> MIIINKNNDKKSLFLLLVSLIFVLFVSNVIADTDYAISPVSLLLPYSTSKYRKPYKLEANKGCFEWINTNPDLVEITPLYESAASCSPSSNDKQQNIGAPDLSLWDNSLNQPNKKCSKAVLVSVRSGTVSERNSAFIYAEEQVTGKKLQCEVFVDRISSIVIETTTKTMYKDDLEELHVRAYDSVGNVFSSIIGLEFEWSITSGNIIQIVPFRGFPLDDVALKMEQESLQTSFVLVQGVDTGRTEINTKLTEPTYKDIQHSTTISILEPLQLNPSYLLYVIPGTQIQYQLLTKKRNILENIPLPNPNYIWSSSNSKVGKVDNSGNFMALDLGRTDLKVQHKNMSDNKVQAFVNVVHPSYLAIKIEPLKSGLGPVSNWNLIENRDYILVVELYDASGHKIHSSEITFDLNIPTEYFERLPSSQIPPNTPKRSDTFYLKAIKQGLVALKASLVKVYDLNLKKYTQLLNPISVEQEVTIHSQIQLSPPIVYLPYLPNHRQYSMIRPIGGSGEYNWYTNNSAIVTVDPTGAITSQTSSGQTEVIVVDKKNPHNRDKVLVIVLQPDEIIITPSQVEVQVGQTLKLSTQLLSKQLSKGVHFDSCNLDDLEWRVDDSNANNDNNGGGGSNQERSFSLLPLQKTNTPKKEQPDLCSTREFLAIKEGSNVISVSYMGMRAKILIFAYPPLKSDQSEILLTLGSTLNVFFSGGPEPWHLERKSHFQSIVSNLTNEQNVLSIVPGNGNSFRVTCLTHTNPSKPIGIELTIGNKVTTTNPYPASPSITIPYSCRPPASIQLQVANLPKDHQIQDSSHHQQIQQQEQQQQQQQQQSTCQDTIFSIKKQKQGEIGTYKIRNDRDIPFIAQVFDDNGKPFTNYSSLVFDWKSSDQTQAKWLRDYNQNDHLSTLSLSKEQGKVIITVSILGYDQELLRQNKIRSSDLDTSKLVSSLELHLLSSVVLFPDYYTMYLNDKNHLKIEAIGGSKNFAFTSNNSKIASLSYQPNSDFVTVIPNQQGYLKVEVRDICLGSDNNKDQQQQYQQKQQKHQQQQQSNTSPSIVQISEVHSIELDVQDMVQVGDSINLIVKGFSQNGQQFDSTQY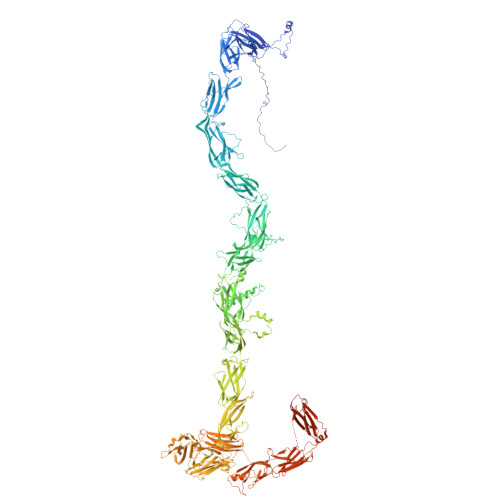QYMNIIPHIDNPNVLSMTQSSDSQVFTLKGLDQGLVTLSVTIQNPKTSFSATSKTIQIQVFPPFRVSPSVLHLVPGGHFQIHWTGGAPIRQDVSFVSSDPSIVNLSGREDLVGELVALKVGEATIKAIAQIVDPITGKKTIIGEDKLMVYVKNMTGIRIHSSINKILVGNEAKLRVVGANGETPFTYGTVDLFFKWECLDSNIATLLPIYERANTTVEAEGSFSVRVMGKNAGSTSITVWAYSGGDKTKHLFQAASLQINVIPDIPIQTTSLLLPLNTPSSFIVNNHLDKTGIEFYPLMDGHGSSSCKDVIDIGDNKIVSLDKIGTCYVSAVRDGRMDTSKLFKINSKPFSHLELLPINPTSTVIPIGGSMSFAIYLRDDIGEVFTEYGSSAIFSSEVSNTGIISSSIDANVVTIKGIRAGLVTLHVYLKDMPHLDDYIKIFVGRLVEPHQPILHVGSMITFSIAKDQLEQRGFSLPSSDEKVWSSGDPSILQVDPITGKATAIAAGTTTINYIRNPSSQTQVVISKIGRIKVDFSDQIINNSKKRYEYNLKFFTAGSDIELSQDSTIDQNIKGICTIKESTFATAFFEKVKGKEQYRCVVQPSGVATSSIDKVTLYVEVSNAHKTYQYDTTINLPFESTFSIINVRDNKIQLSPRQSTFILNIQSSSPIFVESSDNSLLSVQQISSSGGDDQLNNLYKYAIQPMSVSTSFQNVPLLISSADGKSKTTVTVSYSKSGSTTSDQNTSYVESSTINSHPFLFSFIIIVGTLLIGLYASKKHNDKPRVYINPNSNLQTSSISSPYRTPPPHSFTSPNRSTYGSSSIYLNN> MAELRMEHIYKFYDQKEPAVDDFNLHIADKEFIVFVGPSGCGASTTLRMVAGLEEISKGDFYIEGKRVNDVAPKDRDIAMVFQNYALYPHMTVYDNIAFGLKLRKMPKPEIKKRVEEAAKILGLEEYLHRKPKALSGGQRQRVALGRAIVRDAKVFLMDEPLSNLDAKLRVQMRAEIIKLHQRLQTTTIYVTHDQTEALTMATRIVVMKDGKIQQIGTPKDVYEFPENVFVGGFIGSPAMNFFKGKLTDGLIKIGSAALTVPEGKMKVLREKGYIGKEVIFGIRPEDIHDELIVVESYKNSSIKAKI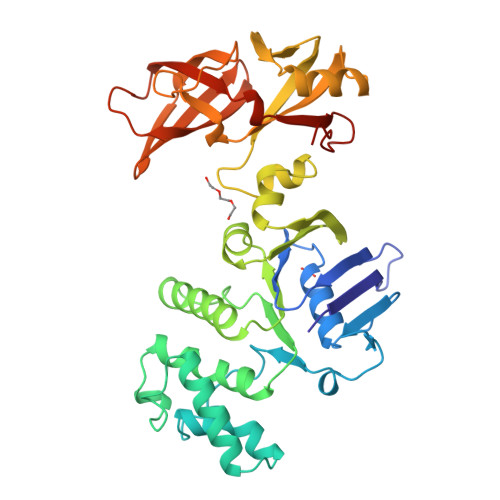NVAELLGSEIMIYSQIDNQDFIARIDARLDIQSGDELTVAFDMNKGHFFDSETEVRIRLEHHHHHH>[2x]TNMSIKEQRESLPVFQFRDQIIQAVKDNQILIVVGETGSGKTTQVTQYLAEAGFTKYGMIGCTQPRRVAAVSVAKRVAEEVGCQLGQEVGYTIRFEDVTSPATKIKYMTDGMLQREILMDPDLKRYSVIMLDEAHERTIATDVLFALLKKTVKRRPDLKVIVTSATLDAEKFSEYFNSCPIFTIPGRTFPVEILYSREPEPDYLEAALTTVMQIHLTEPPGDILVFLTGQEEIDTACEILYERMKALGPSVPELIILPIYSALPSEMQSRIFEPAPPGSRKVVIATNIAETSITIDYIYYVVDPGFVKQNAYDPKLGMDSLVVTP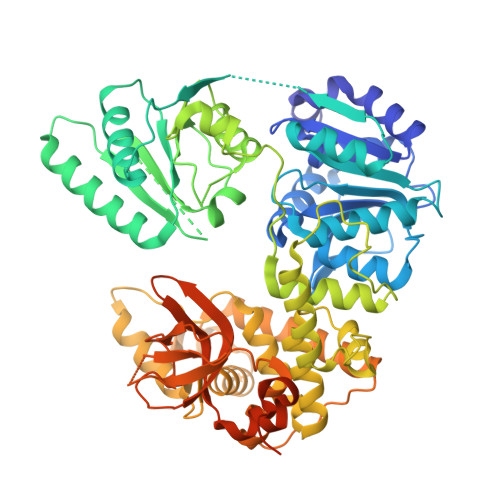ISQAQANQRAGRAGRTGPGKCFRLYTEAAYQSEMLPTTIPDIQRQNLANTILLLKAMGINDLLRFDFMDPPPVNTMLTALEELYALGALDDEGLLTRLGRKMADFPMEPSLSKVLIASVDKGCSDEMVTIVSMLNLQQIFYRPKDKQQQADQKKAKFHDPTGDHLTLLNVYNAWKNSGYSNAWCFENYIQARAMRRARDVRQQIVKIMERHRHPIISCGRDTDKIRQALCAGFFRNTARKDPQEGYKTLTEGTPVYLHPSSALFGKQAEWVLYHELVLTTKEYMHFTTAIEPKWLVEAAPTFFKLAPTDRLSKRKKAERIQPLYNKYEGEDGWRLSAQRRAARPGGGGGTWG>MMMKKGLLAGALTATVLFGTCAVDAPGIISPKTAEAASQLTDGIGGRAYLNSTGAIFVTKIQLPSSIQVSNGTAYIYSGFSGGTESDIGFQYSDKYNVWKPYMKVGSKGQDQVQYLEGGSQFTNTKGFRPGSTVQLTIYKNLNGNTRATYWGTNNAGYNGRLISEISKTNVGSISKW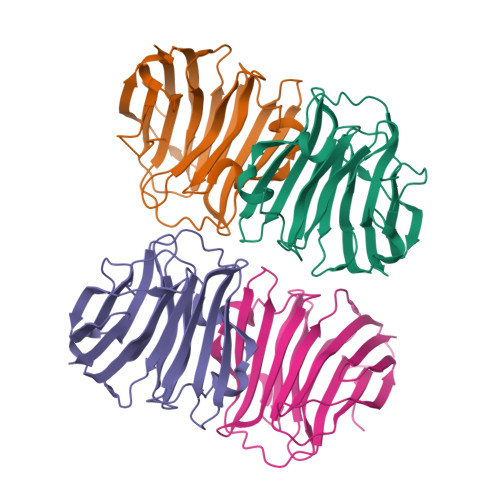KALATVATTGSRQSIKSNFSTSFTNITIDNKAITPVIDTQDFAKVTVSGNSVSLSVVKN[4x]>MSEMSSFLHIGDIVSLYAEGSVNGFISTLGLVDDRCVVEPAAGDLDNPPKKFRDCLFKVCPMNRYSAQKQYWKAKQTKQDKEKIADVVLLQKLQHAAQMEQKQNDTENKKVHGDVVKYGSVIQLLHMKSNKYLTVNKRLPALLEKNAMRVTLDATGNEGSWLFIQPFWKLRSNGDNVVVGDKVILNPVNAGQPLHASNYELSDNAGCKEVNSVNCNTSWKINLFMQFRDHLEEVLKGGDVVRLFHAEQEKFLTCDEYKGKLQVFLRTTLRQSATSATSSNALWEVEVVHHDPCRGGAGHWNGLYRFKHLATGNYLAAEENPSYKGDASDPKAAGMGAQGRTGRRNAGEKIKYCLVAVPHGNDIASLFELDPTTLQKTDSFVPRNSYVRLRHLCTNTWIQSTNVPIDIEEERPIRLMLGTCPTKEDKEAFAIVSVPVSEIRDLDFANDASSMLASAVEKLNEGFISQNDRRFVIQLLEDLVFFVSDVPNNGQNVLDIMVTKPNRERQKLMREQNILKQVFGILKAPFREKGGEGPLVRLEELSDQKNAPYQHMFRLCYRVLRHSQEDYRKNQEHIAKQFGMMQSQIGYDILAEDTITALLHNNRKLLEKHITKTEVETFVSLVRKNREPRFLDYLSDLCVSNHIAIPVTQELICKCVLDPKNSDILIRTELRPVKEMAQSHEYLSIEYSEEEVWLTWTDKNNEHHEKSVRQLAQEARAGNAHDENVLSYYRYQLKLFARMCLDRQYLAIDEISQQLGVDLIFLCMADEMLPFDLRASFCHLMLHVHVDRDPQELVTPVKFARLWTEIPTAITIKDYDSNLNASRDDKKNKFANTMEFVEDYLNNVVSEAVPFANEEKNKLTFEVVSLAHNLIYFGFYSFSELLRLTRTLLGIIDCVQGPPAMLQAYEDPGGKNVRRSIQGVGHMMSTMVLSRKQSVFSAPSLSAGASAAEPLDRSKFEENEDIVVMETKLKILEILQFILNVRLDYRISYLLSVFKKEFVEVFPMQDSGADGTAPAFDSTTANMNLDRIGEQAEAMFGVGKTSSMLEVDDEGGRMFLRVLIHLTMHDYAPLVSGALQLLFKHFSQRQEAMHTFKQVQLLISAQDVENYKVIKSELDRLRTMVEKSELWVDKKGSGKGEEVEAGAAKDKKERPTDEEGFLHPPGEKSSENYQIVKGILERLNKMCGVGEQMRKKQQRLLKNMDAHKVMLDLLQIPYDKGDAKMMEILRYTHQFLQKFCAGNPGNQALLHKHLHLFLTPGLLEAETMQHIFLNNYQLCSEISEPVLQHFVHLLATHGRHVQYLDFLHTVIKAEGKYVKKCQDMIMTELTNAGDDVVVFYNDKASLAHLLDMMKAARDGVEDHSPLMYHISLVDLLAACAEGKNVYTEIKCTSLLPLEDVVSVVTHEDCITEVKMAYVNFVNHCYVDTEVEMKEIYTSNHIWTLFENFTLDMARVCSKREKRVADPTLEKYVLSVVLDTINAFFSSPFSENSTSLQTHQTIVVQLLQSTTRLLECPWLQQQHKGSVEACIRTLAMVAKGRAILLPMDLDAHISSMLSSGASCAAAAQRNASSYKATTRAFPRVTPTANQWDYKNIIEKLQDIITALEERLKPLVQAELSVLVDVLHWPELLFLEGSEAYQRCESGGFLSKLIQHTKDLMESEEKLCIKVLRTLQQMLLKKTKYGDRGNQLRKMLLQNYLQNRKSTSRGDLPDPIGTGLDPDWSAIAATQCRLDKEGATKLVCDLITSTKNEKIFQESIGLAIHLLDGGNTEIQKSFHNLMMSDKKSERFFKVLHDRMKRAQQETKSTVAVNMNDLGSQPHEDREPVDPTTKGRVASFSIPGSSSRYSLGPSLRRGHEVSERVQSSEMGTSVLIMQPILRFLQLLCENHNRDLQNFLRCQNNKTNYNLVCETLQFLDIMCGSTTGGLGLLGLYINEDNVGLVIQTLETLTEYCQGPCHENQTCIVTHESNGIDIITALILNDISPLCKYRMDLVLQLKDNASKLLLALMESRHDSENAERILISLRPQELVDVIKKAYLQEEERENSEVSPREVGHNIYILALQLSRHNKQLQHLLKPVKRIQEEEAEGISSMLSLNNKQLSQMLKSSAPAQEE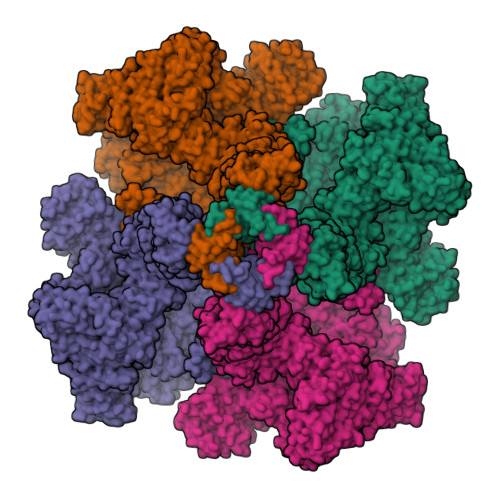EEDPLAYYENHTSQIEIVRQDRSMEQIVFPVPGICQFLTEETKHRLFTTTEQDEQGSKVSDFFDQSSFLHNEMEWQRKLRSMPLIYWFSRRMTLWGSISFNLAVFINIIIAFFYPYMEGASTGVLDSPLISLLFWILICFSIAALFTKRYSIRPLIVALILRSIYYLGIGPTLNILGALNLTNKIVFVVSFVGNRGTFIRGYKAMVMDMEFLYHVGYILTSVLGLFAHELFYSILLFDLIYREETLFNVIKSVTRNGRSILLTALLALILVYLFSIVGFLFLKDDFILEVDRLPNNHSTASPLGMPHGAAAFVDTCSGDKMDCVSGLSVPEVLEEDRELDSTERACDTLLMCIVTVMNHGLRNGGGVGDILRKPSKDESLFPARVVYDLLFFFIVIIIVLNLIFGVIIDTFADLRSEKQKKEEILKTTCFICGLERDKFDNKTVSFEEHIKLEHNMWNYLYFIVLVRVKNKTDYTGPESYVAQMIKNKNLDWFPRMRAMSLVXXXXXXXXXXXXXXXXXXXXXX[4x]> AKPVPPPR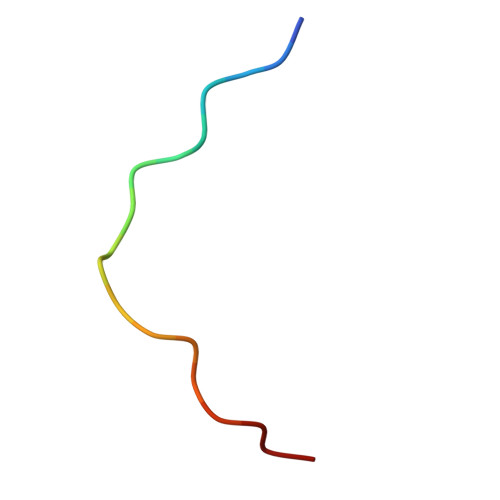GAKPAPPPRT> MTESPTTHHGAAPPDSVATPVRPWSEFRLTPAEAAAAAALAARCAQRYDETDGPEFLLDAPVIAHELPRRLRTFMARARLDAWPHALVVRGNPVDDAALGSTPVHWRTARTPGSRPLSFLLMLYAGLLGDVFGWATQQDGRVVTDVLPIKGGEHTLVSSSSRQELGWHTEDAFSPYRADYVGLLSLRNPDGVATTLAGVPLDDLDERTLDVLFQERFLIRPDDSHLQVNNSTAQQGRVEFEGIAQAADRPEPVAILTGHRAAPHLRVDGDFSAPAEGDEEAAAALGTLRKLIDASLYELVLDQGDVAFIDNRRAVHGRRAFQPRYDGRDRWLKRINITRDLHRSRKAWAGDSRVLGQR

The utility of the method is highlighted by studies with three X-ray-radiation-sensitive Fe(II)-containing model enzymes: the 2-oxoglutarate-dependent l-arginine hy­droxy­lase VioC and the DNA repair enzyme AlkB, as well as the oxidase isopenicillin N synthase (IPNS), which is involved in the biosynthesis of all penicillin and cephalosporin antibiotics. However, maintaining an anaerobic environment for di­oxy­gen-dependent enzymes has not been explored for serial room-temperature data collection at synchrotron light sources. This work describes a methodology that employs an adaptation of the ‘sheet-on-sheet’ sample mount, which is suitable for the low-dose room-temperature data collection of anaerobic samples at synchrotron light sources. As demonstrated by the lack of turnover observed with two 2OG oxygenases and IPNS, our method slows di­oxy­gen penetration to a level that enables data collection within a reasonable timeframe.

(1) VioC (Streptomyces vinaceus) is a 2OG-dependent l-arginine hy­droxy­lase that catalyses the production of (3S)-hy­droxy­arginine from l-arginine and which is involved in the biosynthesis of tuberactin antibiotics (e.g. viomycin) which have been used to treat Mycobacterium tuberculosis infections. Importantly, clear differences in the active sites of the two structures were observed, with apparently complete conversion of 2OG to succinate and carbon dioxide (not observed), and of arginine to (3S)-hydroxy­arginine in the air-exposed structure. The non-metal-ion ligating co-substrate/co-product carboxyl­ate is positioned to interact with the guanidinium group of Arg330 via a salt bridge. Binding of both the arginine substrate and the 3-hy­droxy­arginine product in VioC is characterized by interactions with Asp270 (with the substrate/product guanidino group), Ser224 and Ser156 (with the substrate/product carboxyl­ate group), and via a hydrogen bond between Glu170 (part of the 2-His-1-carboxyl­ate triad) and the α-amino group of the substrate/product. Structures of VioC in complex with arginine solved under cryo-conditions have revealed a second conformation of the substrate, which we did not observe in our structure, probably due to its lower resolution.>SNAMKILVTSGGTSEAIDSVRSITNHSTGHLGKIITETLLSAGYEVCLITTKRALKPEPHPNLSIREITNTKDLLIEMQERVQDYQVLIHSMAVSDYTPVYMTGLEEVQASSNLKEFLSKQNHQAKISSTDEVQVLFLKKTPKIISLVKEWNPTIHLIGFKLLVDVTEDH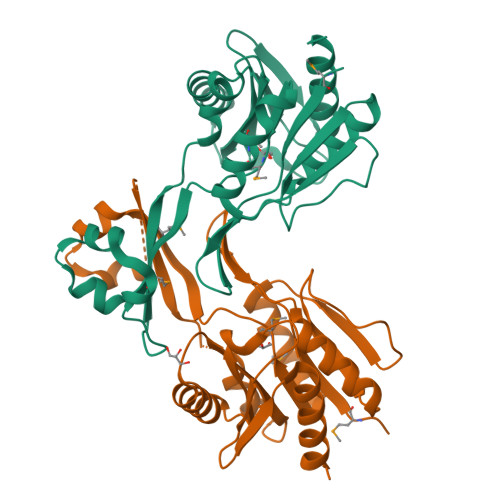LVDIARKSLIKNQADLIIANDLTQISADQHRAIFVEKNQLQTVQTKEEIAELLLEKIQAYHS[2x]> MNQQKSLTLIVALTTSYGIGRSNSLPWKLKKEISYFKRVTSFVPTFDSFESMNVVLMGRKTWESIPLQFRPLKGRINVVITRNESLDLGNGIHSAKSLDHALELLYRTYGSESSVQINRIFVIGGAQLYKAAMDHPKLDRIMATIIYKDIHCDVFFPLKFRDKEWSSVWKKEKHSDLESWVGTKVPHGKINE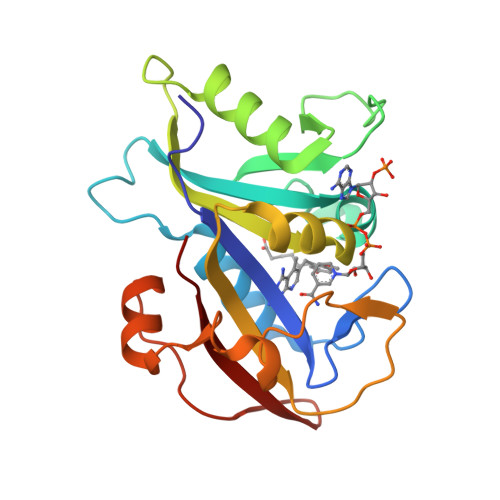DGFDYEFEMWTRDL>[2x]GSAMGSKPAKPLPKEMEEFVQSSGENGVVVFSLGSMVS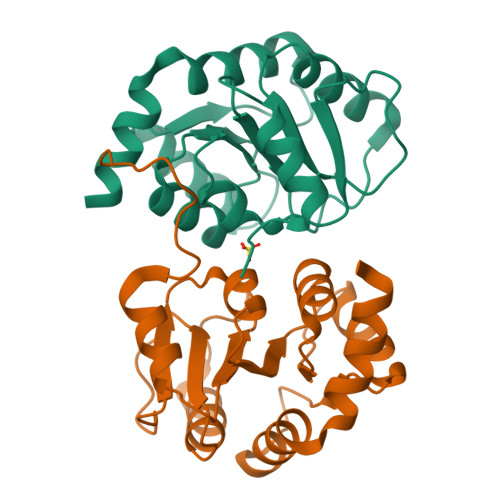NMTEERANVIATALAKIPQKVLWRFDGNKPDALGLNTRLYKWIPQNDLLGHPKTRAFITHGGANGIYEAIYHGIPMVGIPLFFDQPDNIAHMKAKGAAVRVDFNTMSSTDLLNALKTVINDPSYKENIMKLSRIQH>[2x]AEPQPASSGLTDETAFSCCSDPDPSTKDFLLQQTMLRIKDPKKSLDFYTRVLGLTLLQKLDFPAMKF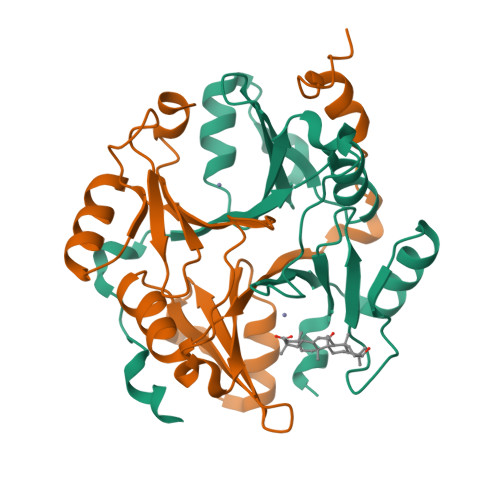SLYFLAYEDKNDIPKDKSEKTAWTFSRKATLELTHNWGTEDDETQSYHNGNSDPRGFGHIGIAVPDVYSACKRFEELGVKFVKKPDDGKMKGLAFIQDPDGYWIEILNPNKIATII>MGGLDTVYEIAAKRLAELGDEESLAELEEYYKTFKKKLKEGTISETTAANSLAIMATRLLERAREKAHHHHH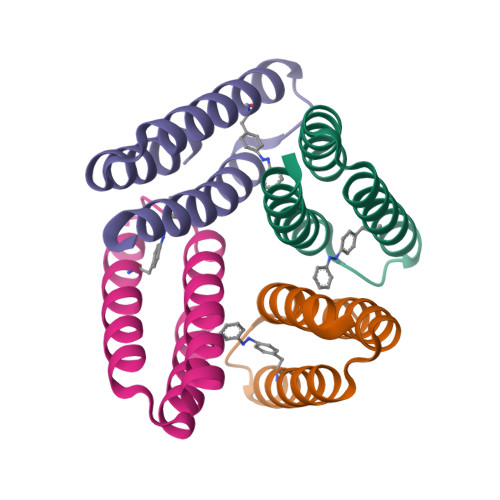H[4x]> XASQDQVDD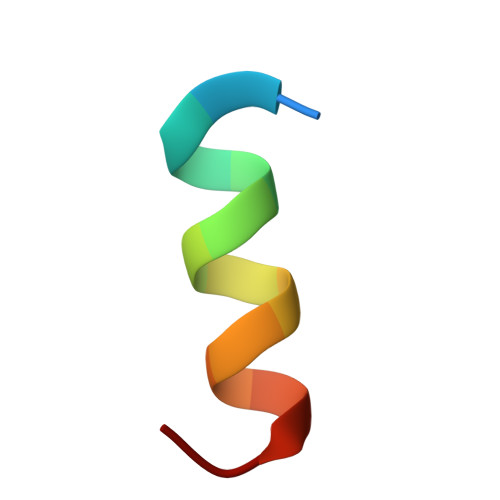LLDSLGF>MQEFEFAVPAPSRVSPDLARARARHLDWVHAMDLVRGEEARRRYEFSCVADIGAYGYPHATGADLDLCVDVLGWTFLFDDQFDAGDGRERDALAVCAELTDLLWKGTAATAASPPIVVAFSDCWERMRAGMSDAWRRRTVHEWVDYLAGWPTKLADRAHGAVLDPAAHLRARHRTICCRPLFALAERVGGYEVPRRAWHSSRLDGMRFTTSDAVIGMNELHSFEKDRAQGHANLVLSLVHHGGLTGPEAVTRVCDLVQGSIESFLRL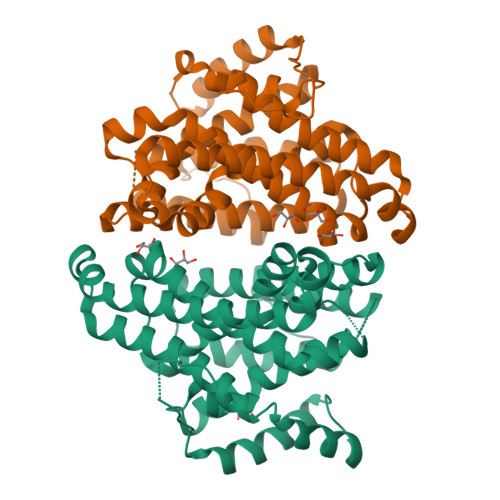RSGLPELGRALGVEGAVLDRYADALSAFCRGYHDWGRGASRYTTRDHPGDLGLENLVARSSG[2x]>STAGKVIKCKAAVLWEVKKPFSIEDVEVAPPKAYEVRIKMVAVGICRTDDHVVSGNLVTPLPVILGHEAAGIVESVGEGVTTVKPGDKVIPLFTPQCGKCRVCKNPESNYCLKNDLGNPRGTLQDGTRRFTCRGKPIHHFLGTSTFSQYTVVDENAVAKIDAASPLEKVCLIGCGFSTGYGSAVNVAKVTPGSTCAVFGLGGVGLSAVMGCKAAGAARIIAVDINKDKFAKAKELGATECINPQDYKKPIQ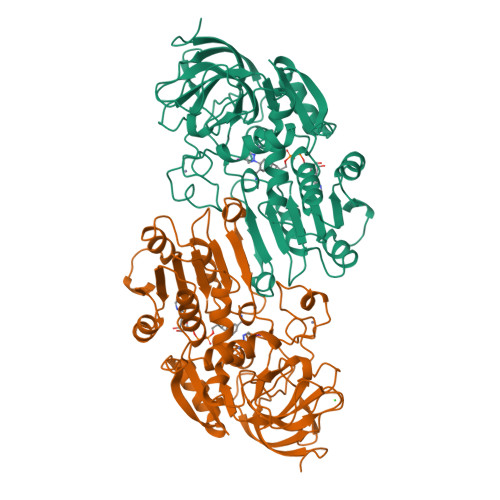EVLKEMTDGGVDFSFEVIGRLDTMMASLLCCHEACGTSVIVGVPPASQNLSINPMLLLTGRTWKGAVYGGFKSKEGIPKLVADFMAKKFSLDALITHVLPFEKINEGFDLLHSGKSICTVLTF[2x]>HMMNRIKKVLVANRGEIAIRVMRACTELKIKTVAIYSQEDTGSFHRYKSDEAYLVGAGKKPIDAYLDIENIIEIAKESGADAIHPGYGFLSENIEFARRCEQEGIIFVGPKSKHLDMFGDKIKAKEQALLADIPVIPGSNGPVAGIKEVEEFGEKNGYPLMIKASLGGGGRGMRVVESKEHVKESFERASSEAKAAFGNDEVYVEKCVMNPKHIEVQILGDTHGNIVHLFERDCSIQRRHQKVVEVAPCNAITSELRNRICDAAVKLMKNVDYINAGTVEFLVEGDDFYFIEVNPRVQVEHTITEMITGIDIVQSQLFIADGYALHDQLVAIPKQEDIHIHGSAIQSRITTEDPLNNFMPDTGRVDTYRSTGGFGVRLDAGNGFQGTVVTPFYDSLLVKLCTWGMTFEQATRKMRRNLIEFRIRGVKTNIPFLLNVVRHPDFASGNYNTSFIDTTPELFKFPHIRDRGTKTLRYIGNVTVNGFPGIKHRDKPVYAEPRLPKIPYGSQISPGTKQILDAKGPEGVVDWVKKQEEVLLTDTTLRDAHQSLLATRVRSKDIFQIADAMAHLLPNMFSFEMW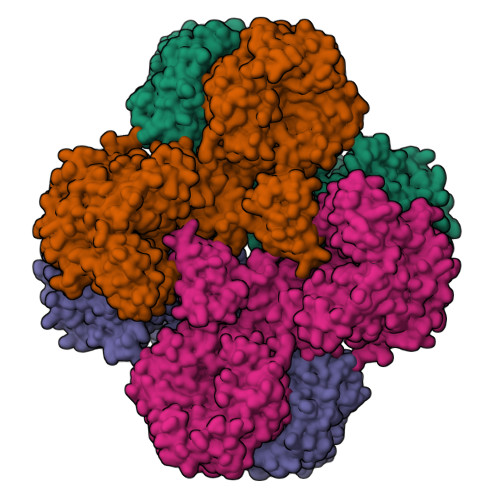GGATFDVAYRFLNEDPWVRLETLRKQIPNVMFQMLLRGANAVGYKNYPDNVIREFVKQSAQSGVDVFRVFDSLNWIKGMEVSIDAVREAGKIVEAAICYTGDIDDDTRTKYTIDYYKDMAKELVAQGTHILGIKDMAGLLKPQAAYRLIGELKDTVDVPIHLHTHDTSGNGIYTYAAAVSAGVDIVDVASSAMSGATSQPSMTGLYYGLVNGNRQTNLDAQNSQIINHYWEDVRHYYKDFDNALNSPQTEVYIHEMPGGQYTNLQQQAIAVGLGDRWDEVKEMYTVVNQMFGDIVKVTPSSKVVGDLALFMVQNELSEEDVYEKGDTIDFPDSVIEFFMGEIGQPYGGFPEKLQKLVLKGRTPLTDRPGALMEPVNFVEVKAELKEKMGYEPTEKDVISYILYPKVFLDYQEMINKYGDVTVLDTPTFYKGMRLGETIEVELEKGKILLIKLNSIGEPIADGTRVIYFELNGQPREINIQDMNVQSTVIARRKIDTTNPEHVGATMTGSVIQVVVKKGDSVKKGDPLLITEAMKMETTIQAPFDGEVSSIYVSDGDTIESGDLLIEVNRI[4x]> GAMNAQAEEFKKYLETNGIKPKQFHKKELIFNQWDPQEYCIFLYDGITKLTSISENGTIMNLQYYKGAFVIMSGFIDTETSVGYYNLEVISEQATAYVIKINELKELLSKNLTHFFY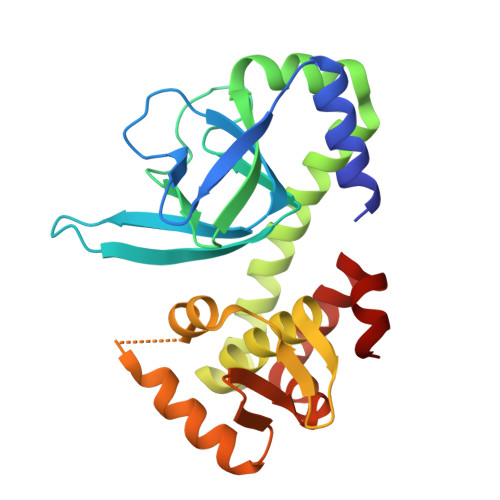VFQTLQKQVSYSLAKFNDFSINGKLGSICGQLLILTYVYGKETPDGIKITLDNLTMQELGYSSGIAHSSAVSRIISKLKQEKVIVYKNSCFYVQNLDYLKRYAPKLDEWFYLACPATWGKLN>[2x]MQRRHFLKNAAAALAALGLPALPPWALAAKAVGLRRLGQPQPFDYAWLKGQARALAKAPYKSHKQVLPGPLESLNWDQYQSIRYRQDHALWADGNGKFQAKFFHLGLYFHTPVHIYDIVDGKAQQLAYDPAAFDYGRSGLGGKQLPKDLGFAGFRLNTRKDTDRDFSAFLGASYFRAVGKEGQYGQSARGLAIDTGTGGPEEFPDFIAYYLEQPADDSDTVVVYGLLDSPSVSGAYRFAITNGEVLVMDIDSALYPRKAIERLGIGPCTSMYQTGENDRRMDWDWRPEIHDTDGLAMWTG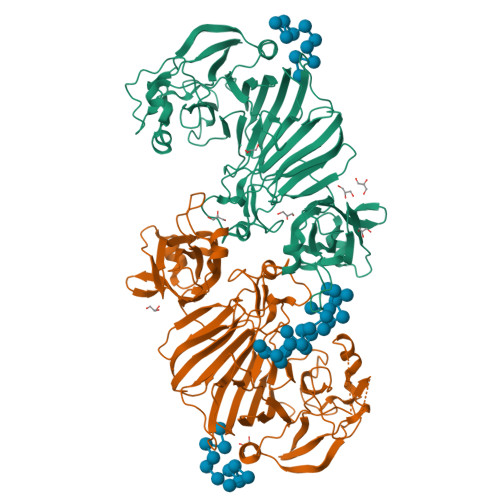GGEWIWRPLCNPPHLRFNMFVDENPRGFGLLQRDRNFDHYQDDGVFYEKRPCLWVEPKSGWGKGSVQLVEIPTVDETFNNIVAFWNPQAKPQPGQELLMGYRLYWGAHPPASSPLAHCVATRTGLGGIVGQKRSHFSWRFAVDFAGGELAALAKDPKAKVEAVLQVSRGTTEIVSARPLHELKGYRAMFDLVPPDEGTQQIDIRLFLRANGKPLTETWLYQWTPPPASERKIYLEHHHHHH> METYVNKLHEGSTYTAAVQYNVLEKDDDPASLTIWVPMFQSSMPADLLIKELANVNILVKQISTPKGPSLRVMINSRSAVLAQMPSKFTICANVSLDERSKLAYDVTTPCEIKACSLTCLKSKNMLTTVKDLTMKTLNPTHDIIALCEFENIVTSKKVIIPTYLRSISVRNKDLNTLENITTTEFKNAITNAKIIPYSGLLLVITVTDNKGAFKYIKPQSQFIVDLGAYLEKESIYYVTTNWKHTATRF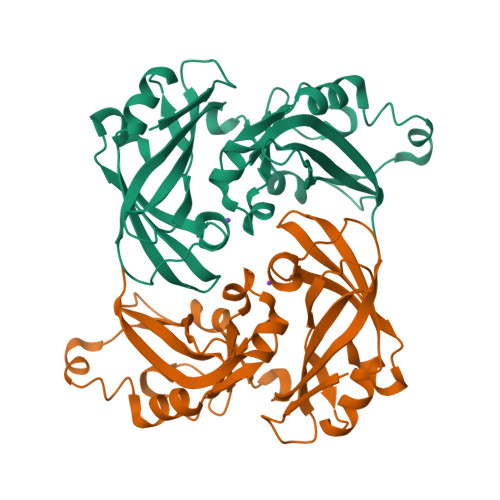AIKPMED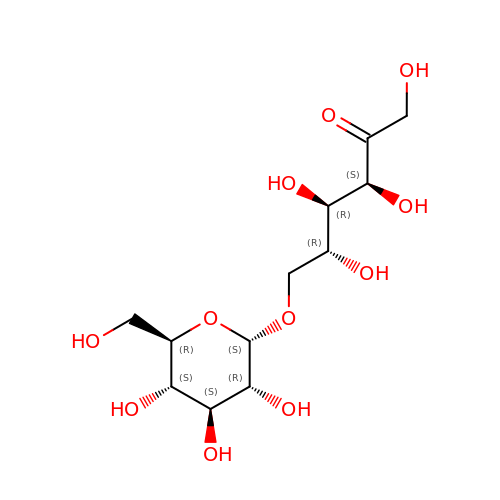6-O-alpha-D-glucopyranosyl-D-fructose | C12 H22 O11 | RJPPRBMGVWEZRR-WTZPKTTFSA-N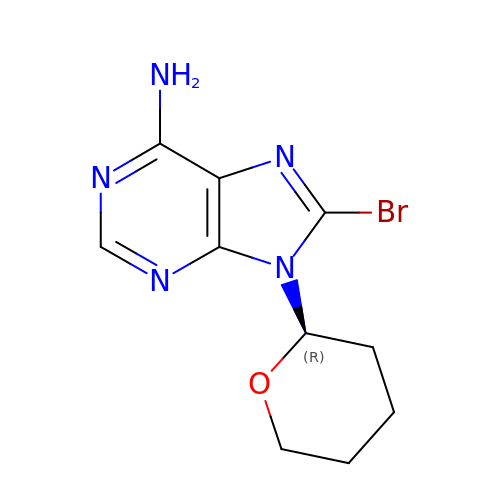8-bromanyl-9-[(2~{R})-oxan-2-yl]purin-6-amine | C10 H12 Br N5 O | FIUISBLUSBJAII-ZCFIWIBFSA-N>GKKCYKLENEKLFEEFLELCKMQTADHPEVVPFLYNRQQRAHSLFLASAEFCNILSRVLSRARSRPAKLYVYINELCTVLKAHSAKKKLN[2x];>VTVDDDDDDNDPENRIAKKMLLEEIKANLS[2x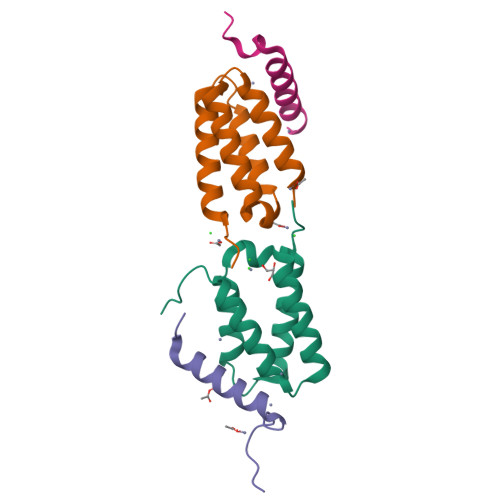]>[3x]MCSTCANVLKYYNWDPHFRLVIDPNKFLSVGFCDNPLMCCYPELLPEFGTVWDCDQSPLQIYLESILGDDEWASTYEAIDPAVPPMHWDAAGKIFQPHPGVLMHHLIGEVAKAWDPNLPMFRLEADGDGSITAPEQGTPVGGVIAEPSAQMSAAADMATGKSVDSEWEAFFSFHTSVNWSTSETQGKILFKQSLGPLLNPYLEHLAKLYVAWSGSIDVRFSISGSGVFGGKLAAIVVPPGVDPVQSTSMLQYPHVLFDARQVEPVIFSIPDLRSTLYHLMSDTDTTSLVIMVYNDLINPYANDSNSSGC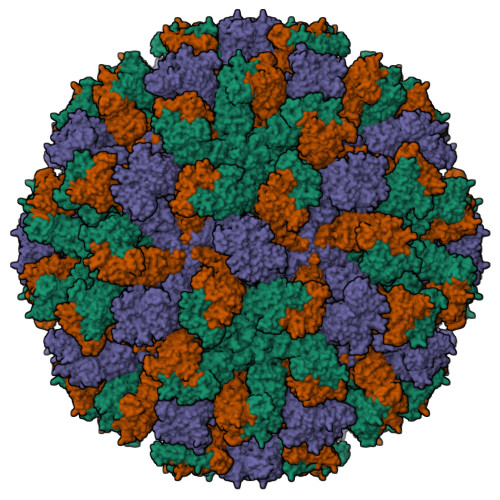IVTVETKPGADFKFHLLKPPGSMLTHGSVPSDLIPKSSSLWIGNRHWTDITDFVIRPFVFQANRHFDFNQETAGWSTPRYRPITITISEKNGAKLGIGVATDYIVPGIPDGWPDTTIPEKLTPAGDYAITNKSGNDITTAAGYDGADVIVNNTNFKGMYICGSLQRAWGDKKISNTAFITTATKVDNAIEPSNVIDMTKIAVYQDTHVGKEVQTSDDTLSLLGYTGIGEQAIGSDRDRVVRISVLPETGARGGNHPIFYKNSIKLGYVIRSIDVFNSQILHTSRQLSLNHYLLPPDSFAVYRIIDSNGSWFDIGIDSDGFSFVGVSSIGKLEFPLTASYMGIQLAKIRLASNIRSSMTKL> GSHMGSPNSPLKDSLRPKLSEEQQHIIAILLDAHHKTYDPTYADFRDFRPPVRMDGSTGSVTLDLSPLSMLPHLADLVSYSIQKVIGFAKMIPGFRDLTSDDQIVLLKSSAIEVIMLRSNQSFTMDDMSWDCGSQDYKYDVTDVSKAGHTLELIEPLIKFQVGLKKLNLHEEEHVLLMAICIVSPDRPGVQDAKLVEAIQDRLSNTLQTYIRCRHPPPGSHQLYAKMIQKLADLRSLNEEHSKQYRSLSFQPENSMKLTPL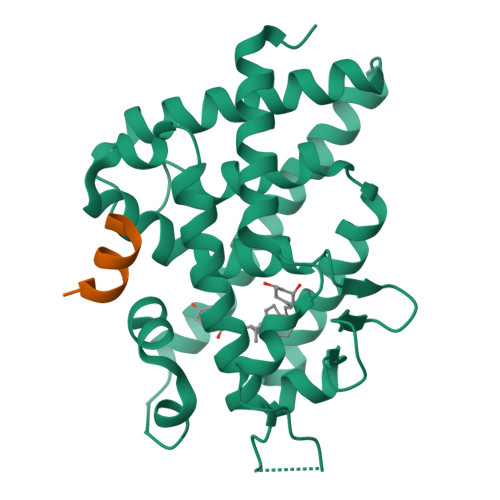VLEVFGNEIS;> KENALLRYLLDKD> SHIEGYECQPIFLNVLEAIEPGVVCAGHDNNQPDSFAALH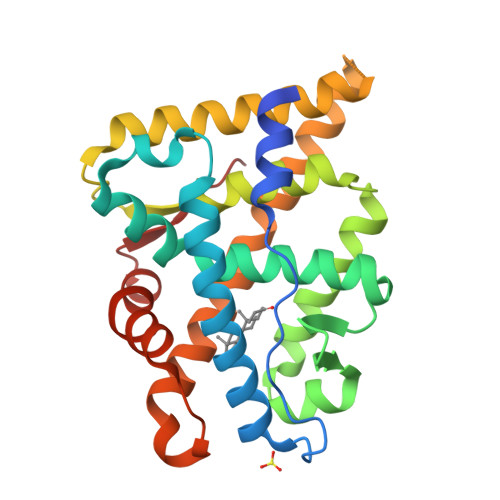SSLNELGERQLVHVVKWAKALPGFRNLHVDDQMAVIQYSWMGLMVFAMGWRSFTNVNSRMLYFAPDLVFNEYRMHKSRMYSQCVRMRHLSQEFGWLQITPQEFLCMKALLLFSIIPVDGLKNQKFFDELRMNYIKELDRIIACKRKNPTSCSRRFYQLTKLLDSVQPIARELYQFTFDLLIKSHMVSVDFPEMMAEIISVQVPKILSGKVKPIYFHTQ(2R)-2-[(3-{3-[(2,4-diamino-6-ethylpyrimidin-5-yl)oxy]propoxy}phenyl)methyl]-3,3-difluoropropanoic 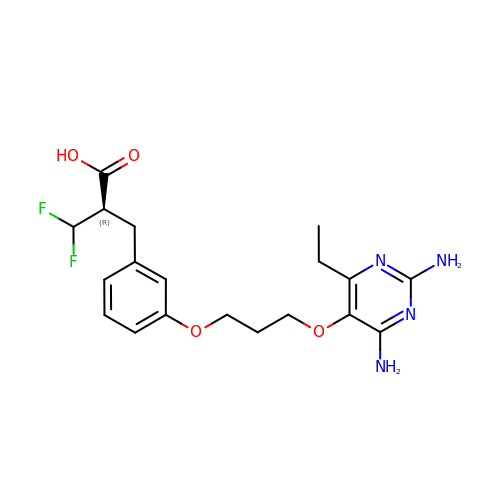acid | C19 H24 F2 N4 O4 | QMHPAIITCHQDEY-ZDUSSCGKSA-N>[2x]GSHMNGLIYAVGGYDGSPDYSTGTHLNSVEAYDPERNEWSLVAPLSTRRSGVGVAVLNGLIYAVGGYDGSPDYSTGTHLN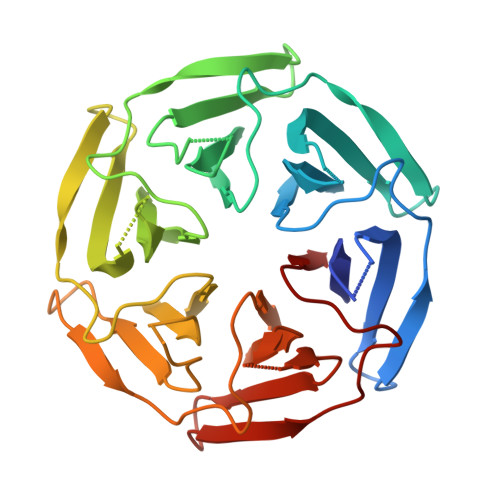SVEAYDPERNEWSLVAPLSTRRSGVGVAVLNGLIYAVGGYDGSPDYSTGTHLNSVEAYDPERNEWSLVAPLSTRRSGVGVAVLNGLIYAVGGYDGSPDYSTGTHLNSVEAYDPERNEWSLVAPLSTRRSGVGVAVLNGLIYAVGGYDGSPDYSTGTHLNSVEAYDPERNEWSLVAPLSTRRSGVGVAVLNGLIYAVGGYDGSPDYSTGTHLNSVEAYDPERNEWSLVAPLSTRRSGVGVAVL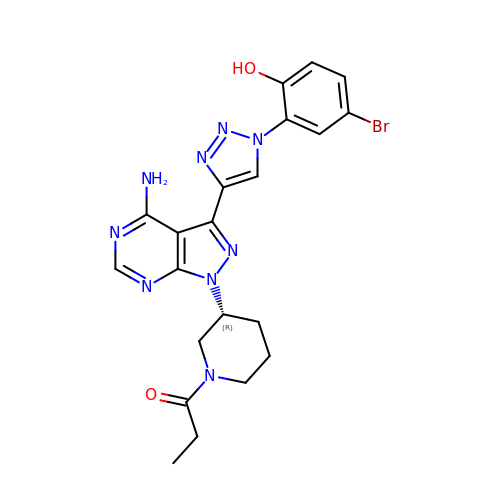1-[(3~{R})-3-[4-azanyl-3-[1-(5-bromanyl-2-oxidanyl-phenyl)-1,2,3-triazol-4-yl]pyrazolo[3,4-d]pyrimidin-1-yl]piperidin-1-yl]propan-1-one | C21 H22 Br N9 O2 | ZXTJFMIWRHTIKC-CYBMUJFWSA-N> MSKTFAEIAEAFLEPEAVRIAKEAVEEYGDHERKIIQIGIHFQVCCMFCDEYLSTNGSDRFVLIEGRKRGTAVSLQNELCKSYDLEPLPFLCDIFDREEKQFVEIGITRKADDSYFQSKFGKLGNSCKIFVFSYDGRLDKNCEGPMEEQKLRIFSFLATAADFLRKENMFNEIFLPDNEETIIEMKKGKTFLELRDESVPLPFQTYEQMKDYCEKFKGNPRELASKVSQMQSNIKLPIKHYEQNKFRQIRLPKGPMAPYTHKFLMEEAWMFTKISDPERSRAGEILIDFFKKGNLSAIRPKDKPLQGKYPIHYKNLWNQIKAAIADRTMVINENDHSEFLGGIGRASKKIPEISLTQDVITTEGLKQSENKLPEPRSFPRWFNAEWMWAIKDSDLTGWVPMAEYPPADNELEDYAEHLNKTMEGVLQGTNCAREMGKCILTVGALMTECRLFPGKIKVVPIYARSKERKSMQEGLPVPSEMDCLFGICVKSKSHLNKDDGMYTIITFEFSI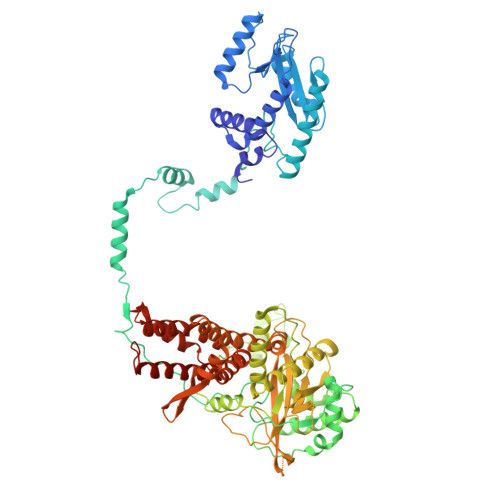REPNLEKHQKYTVFEAGHTTVRMKKGESVIGREVPLYLYCRTTALSKIKNDWLSKARRCFITTMDTVETICLRESAKAEENLVEKTLNEKQMWIGKKNGELIAQPLREALRVQLVQQFYFCIYNDSQLEGFCNEQKKILMALEGDKKNKSSFGFNPEGLLEKIEECLINNPMCLFMAQRLNELVIEASKRGAKFFKTD> MNKPIKNIVIVGGGTAGWMAASYLVRALQQQANITLIESAAIPRIGVGEATIPSLQKVFFDFLGIPEREWMPQVNGAFKAAIKFVNWRKSPDPSRDDHFYHLFGNVPNCDGVPLTHYWLRKREQGFQQPMEYACYPQPGALDGKLAPCLSDGTRQMSHAWHFDAHLVADFLKRWAVERGVNRVVDEVV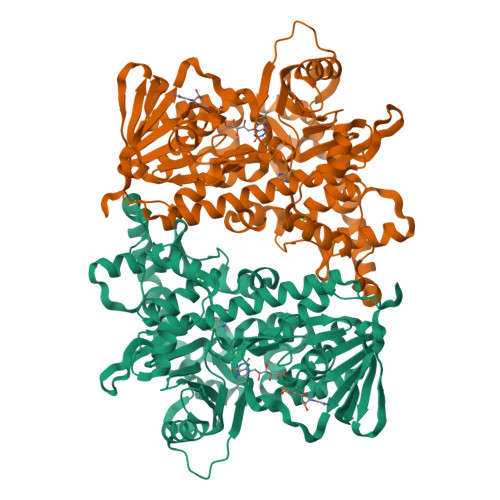DVRLNNRGYISNLLTKEGRTLEADLFIDCSGMRGLLINQALKEPFIDMSDYLLCDSAVASAVPNDDARDGVEPYTSSIAMNSGWTWKIPMLGRFGSGYVFSSHFTSRDQATADFLKLWGLSDNQPLNQIKFRVGRNKRAWVNNCVSIGLSSCFLEPLDSTGIYFIYAALYQLVKHFPDTSFDPRLSDAFNAEIVHMFDDCRDFVQAHYFTTSRDDTPFWLANRHDLRLSDAIKEKVQRYKAGLPLTTTSFDDSTYYETFDYEFKNFWLNGNYYCIFAGLGMLPDRSLPLLQHRPESIEKAEAMFASIRREAERLRTSLPTNYDYLRSLRDGDAGLSRGQRGPKLAAQESL>[2x]MGHHHHHHGGGENLYFQGSMQPDMSLNVIKMKSSDFLESAELDSGGFGKVSLAFHRTQGLMIMKTVYKGPNCIEHNEALLEEAKMMNRLRHSRVVKLLGVIIEEGKYSLVMEYMEKGNLMHVLKAEMSTPLSVKGRIILEIIEGMAYLHGKGVIHKDLKPENILVDNDFHIKIADLGLASFKMWSKLNNEEHNELRE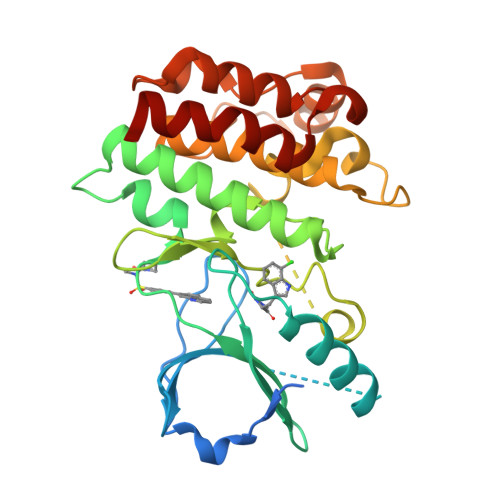VDGTAKKNGGTLYYMAPEHLNDVNAKPTEKSDVYSFAVVLWAIFANKEPYENAIAEQQLIMAIKSGNRPDVDDITEYCPREIISLMKLCWEANPEARPTFPGIEEKFRPFYLSQLE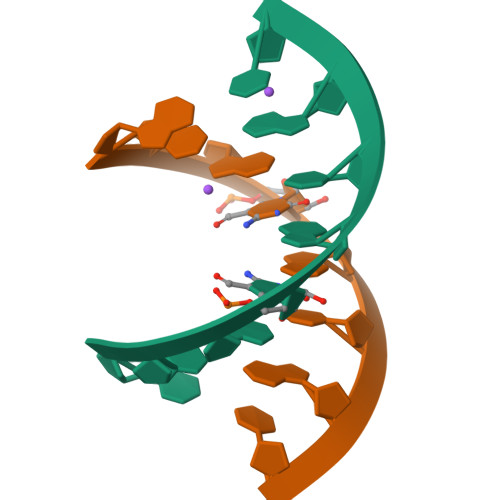>[6x]GUAXGUAC>[2x]MKILVTGAAGFIGSHLCQALLKNSAYHVVGIDHFIGPTPATLKTGNIQSLELNSRFQFIRE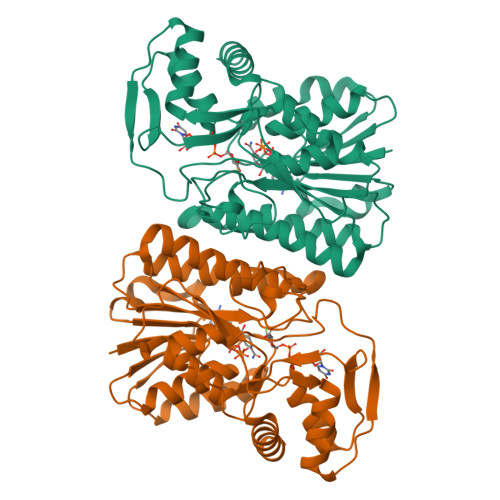DILNTDLSKLLQDIDVVYHLAAIPGVRTSWGKDFQPYVTNNIMVTQQLLEACKHIKLDKFIHISTSSVYGEKSGAVSEDLLPIPLSPFGVTKLSGEHLCHVYHKNFHIPIVILRYFTVYGPRQRPDMAFHRLIKQMLEDKPLTIFGDGTQTRDFTYIDDCIRGTVAALETKKNIIGEVINIGGKEQASILDIISMLEKISGKSATKNFLKSVPGEPKQTWADISKASTLLQYSPTVSLSDGLEAEYDYIKQLYKGDAAWSHPQFEK>[6x]QGHSEEIVLKAGGKIYQGWTKIGITRSLEAMSGAFDLE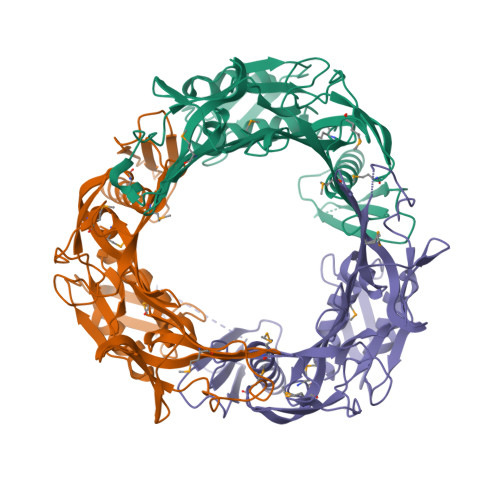MTYKFLGNDAQYKAFIEPIKQGQACTVDIGGERVITGYVDDWVPSYDESTITISVSGRDKTADLVDCSIDYPSGQFNNQTLTQIADIVCKPFGIKVIVNTDVGEPFQRIQIEQGETPHELLARLAKQRGVLLTSDTFGNLVITRASKTKAGVSLILGDNVKAARGRFSWRQRFSKFTIKAAGAAHGQWDSAGLPTVGGIKADVTDSEIGRYRPLIIVNEEVTTAEGAAKRGQWERQRSIGKSNMAEYTVTGWRIPQTGKLWNINTLVPVIDEIMGLDEEMLIASILFSEDDAGRLAVISVVRPDAMDIPAQIVKDTKLGGSTW>MGHHHHHHSHMKWGFRWYGAAGDAIPLKHIRQIPGITGVVGTLLNKLPGDVWTVAEIQALKQSVEQEGLALLGIESVAIHDAIKAGTDQRDHYIDNYRQTLRNLGKCGISLVCYSFKPIFGWAKTDLAYENEDGSLSLLFDQAVVENMQPEDMYQLIHSQSKGFRLPGWEEERLQQFQELKAMYAGVTEEDLVENLRYFLERVIPVCEEENIKMGIHPDDPPWEIFGLPRITKNLADLKRILSLVDSPANGITFCTGSLGADPTNDLPTMIREIGHRINFVHFRNVKYLGEHRFEETAHPSVAGSLDMAELMQA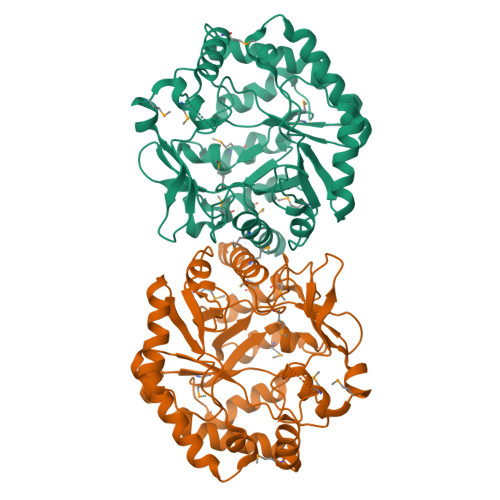LVDVGYEGVIRPDHGRAIWDEKAMPGYGLYDRAMGLTYIQGLYEATKAKQNRK[2x]>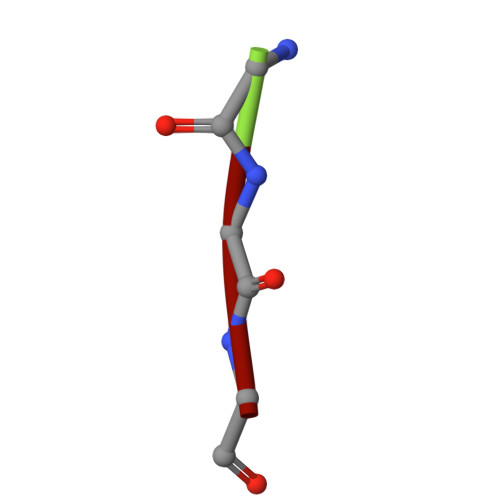 GGG>[2x]WSKCNPLEKTCPPNKGLAASTYTADFTSASALDQWEVTAGKVPVGPQGAEFTVAKQGDAPTIDTDFYFFFGKAEVVMKAAPG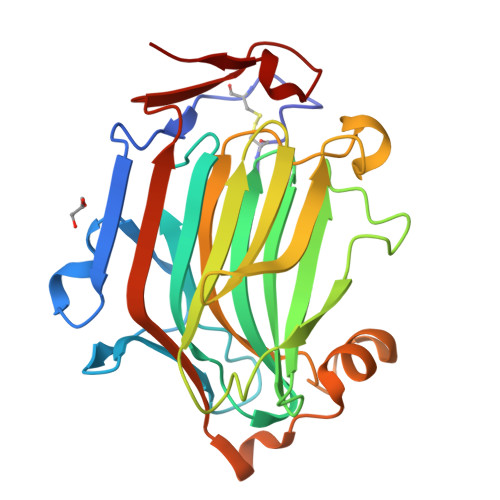TGVVSSIVLESDDLDEVDWEVLGGDTTQVQTNYFGKGDTTTYDRGTYVPVATPQETFHTYTIDWTKDAVTWSIDGAVVRTLTYNDAKGGTRFPQTPMRLRLGSWAGGDPSNPKGTIEWAGGLTDYSAGPYTMYVKSVRIENANPAESYTYSDNSGSWQSIKFD>MDQSVSNVDKSSAFEYNKMIGHGINMGNALEAPVEGSWGVYIEDEYFKIIKERGFDSVRIPIRWSAHISEKYPYEIDKFFLDRVKHVVDVALKNDLVVIINCHHFEELYQAPDKYGPVLVEIWKQVAQAFKDYPDKLFFEIFNEPAQNLTPTKWNELYPKVLGEIRKTNPSRIVIIDVPNWSNYSYVRELKLVDDKNIIVSFHYYEPFNFTHQGAEWVSPTLPIGVKWEGKDWEVEQIRNHFKYVSEWAKKNNVPIFLGEFGAYSKADMESRV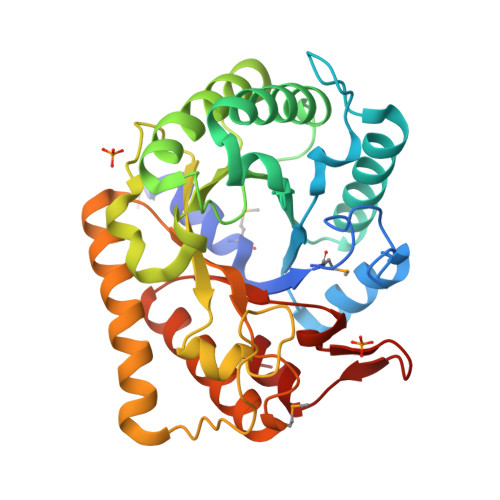KWTKTVRRIAEEFGFSLAYWEFCAGFGLYDRWTKTWIEPLTTSALGK[2x];> ANE;> ADQ> FFDVPAEEDPEVHLGQLKRFSLREL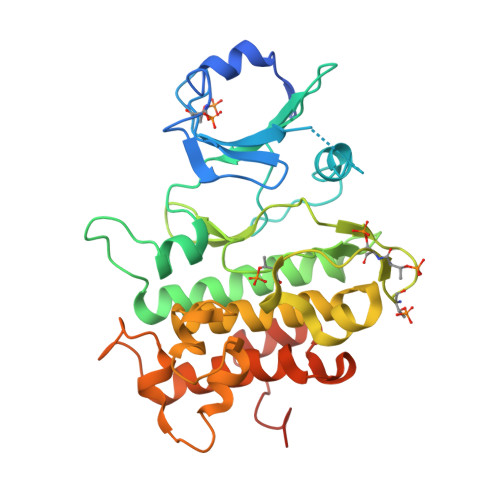QVASDNFSNKNILGRGGFGKVYKGRLADGTLVAVKRLKEERTQGGELQFQTEVEMISMAVHRNLLRLRGFCMTPTERLLVYPYMANGSVASCLRERPESQPPLDWPKRQRIALGSARGLAYLHDHCDPKIIHRDVKAANILLDEEFEAVVGDFGLAKLMDYKDTHVTTAVRGTIGHIAPEYLSTGKSSEKTDVFGYGVMLLELITGQRAFDLARLANDDDVMLLDWVKGLLKEKKLEALVDVDLQGNYKDEEVEQLIQVALLCTQSSPMERPKMSEVVRMLEGDGLAERWEEWQKEEMFRQ>[12x]MGSSHHHHHHSQDLDEVDAGSM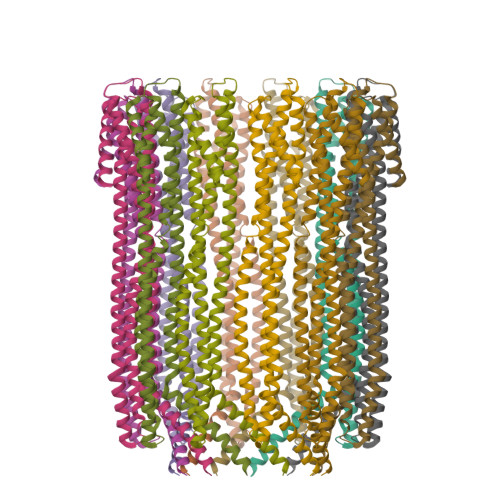TEIVADKTVEVVKNAIETADGALDLYNKYLDQVIPWQTFDETIKELSRFKQEYSQAASVLVGDIKTLLMDSQDKYFEATQTVYEWCGVATQLLAAYILLFDEYNEKKASAQKDILIKVLDDGITKLNEAQKSLLVSSQSFNNASGKLLALDSQLTNDFSEKSSYFQSQVDKIRKEAYAGAAAGVVAGPFGLIISYSIAAGVVEGKLIPELKNKLKSVQNFFTTLSNTVKQANKDIDAAKLKLTTEIVAIGEIKTETETTRFYVDYDDLMLSLLKEAAKKMINTCNEYQKRHGKKTLFEVPEV> GMKQMNVVLIGGGTGLSVLARGLREFPIDITAIVTVADNGGSTGKIRDVMDIPAPGDIRNVIAALSDSESILTQLFQYRFGENQVDGHSLGNLVIAGMTNITNDFGHAIKELSKVLNIKGQVIPSTNASVQLNAVMEDGEIVHGETNIPKTHKKIDRVFLEPSDVEP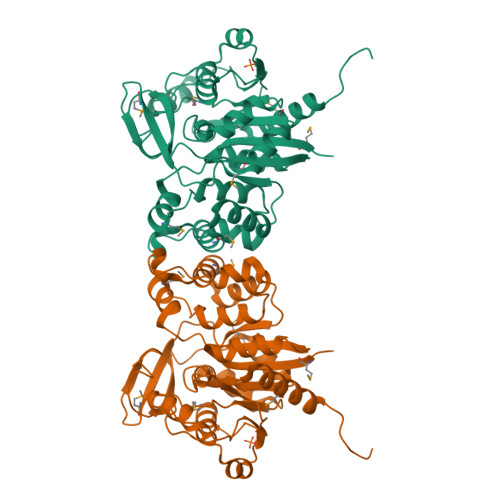MNEAIEALEQADLIVLGPGSLYTSVISNLCVKGISEALLRTSAPKLYVSNVMTQPGETDNYDVKEHIDALTRQVGEPFIDFVICSSESYSKDVLQRYEEKNSKPVAVHKEQLKDSGIRVLTASNLVEISNEHYVRHNTKVLSKMIYELALELTSTIRFTPSDKKK Crenarchaea, one of the two major phyla of cultured archaea, possesses a number of small and basic chromatin proteins, including Sul7d, CC1 and Cren7. In Sulfolobus solfataricus P2, a model strain of Crenarchaeota, Cren7 is synthesized in abundance, constituting ~1% of the total cellular proteins. This protein preferentially binds dsDNA over ssDNA and changes the DNA geometry in vitro. Similar to other Cren7-DNA complexes reported previously, Cren7 binds to the mismatched DNA duplex in the minor groove as a monomer, covering almost all the eight base pairs.

Meanwhile, two complexes are in the asymmetric unit of Cren7-GTGATCGC, which are related by a perfect non-crystallographic 2-fold symmetry axis with a root-mean-square deviation (RMSD) value of 0.018 Å between them. By contrast, both T:G mispairs in the GC-rich DNA duplex (GTGATCGC) retained classic wobble type. To learn more about the atomic details of the unusual T2:G15 base pairing, the structures of all the T:G mispairs in the Cren7-DNA complexes are compared. Both T:G base pairs in the Cren7-GTGATCGC complex form a classic wobble pair with hydrogen bonds from G-O6 to T-N3 (2.74 Å for G7:T10 and 2.72 Å for G15:T2) and from G-N1 to T-O2 (2.91 Å for G7:T10 and 2.83 Å for G15:T2). The bound Cren7 induces a sharp kink (~50°) to the major groove by the intercalation of the side chain of Leu28 into the A3A4 step of d(GTAATTGC)2, while a smaller kink (~48°) is observed at the G3A4 step for d(GTGATCGC)2. The average conformational parameters of the base pair steps in GTGATCGC resembles those in GCGATCGC bound by Cren7. It suggests that the existence of T:G mispairs has little effects on the conformation of GC-rich DNA bound by Cren7. A similar case is found for GTGATCGC, with the values of the corresponding steps being about 15.4°and 18.8°, respectively. Cren7 showed a 1.3-fold reduction in the binding affinity for GTGATCGC as compared to that for GCGATCGC. This was resulted from the combined effects of a slightly decreased association rate (ka) and a slightly increased dissociation rate (kd), indicating that the presence of T:G wobble base pairs had limited effects on both Cren7-DNA contacts and the stability of Cren7-DNA complex. Although predictions based on pairing of the complementary bases and the stacking of pairs suggested no obvious sequence dependent base pair opening probabilities, Cren7 may prefer to induce the opening of T:G base pair in the AT-rich DNA sequences, as the fact that both T:G base pairs in the Cren7-GTGATCGC complex retain the classic wobble type.

>[2x]MSSGKKPVKVKTPAGKEAELVPEKVWALAPKGRKGVKIGLFKDPETGKYFRHKLPDDYPI> MPFEVVFDGAKEFADLIATASNLIDEAAFKFTEEGISMRAMDPSRVVLIDLNLPESIFSKYEVEEPETIGINMDQFKKILKRGKAKDTLILRKGDENFLEITFEGTAKRTFRLPLIDVEELELELPELPFTAKVVL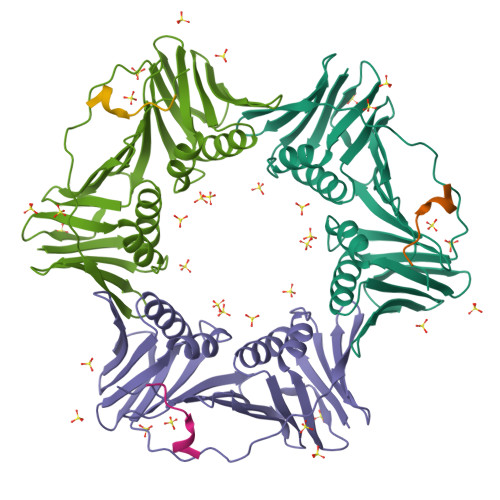LGEVLKEGIKDASLVSDAIKFIAKENEFTMKAEGETNEVEIRLTLEDEGLLDLEVEEETKSAYGIRYLSDMVKGIGKADEVILRFGNEMPLQMEYMIRDEGRLTFLLAPRVEEHHHHHH;> KQRTLESWFGR> LPTSNPAQELEARQLGRTTRDDLINGNSASCADVIFIYARGSTETGNLGTLGPSIASNLESAFGKDGVWIQGVGGAYRATLGDNALPRGTSSAAIREMLGLFQQANTKCPDATLIAGGY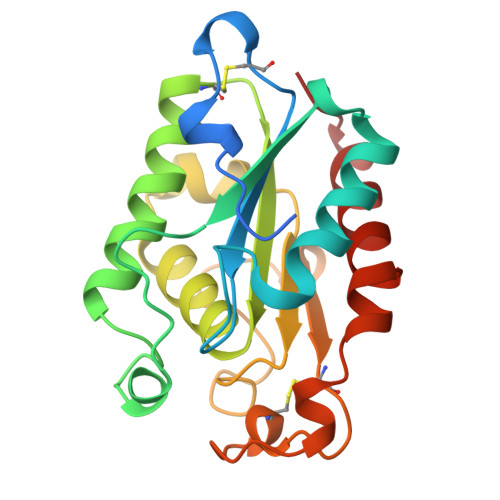AQGAALAAASIEDLDSAIRDKIAGTVLFGYTKNLQNRGRIPNYPADRTKVFCNTGDLVCTGSLIVAAPHLAYGPDARGPAPEFLIEKVRAVRGSA(3~{S},4~{S})-4-(4-pyridin-2-yl-1,2,3-triazol-1-yl)piperidin-3-ol | C12 H15 N5 O | 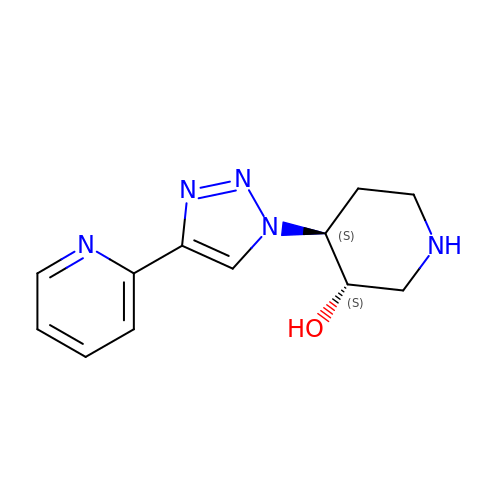HOLBWWKPFXUQIH-RYUDHWBXSA-N>GSHMQQWVDCEFTGRDFRDEDLSRLHTERAMFSECDFSGVNLAESQHRGSAFRNCTFERTTLWHSTFAQCSMLGSVFVACRLRPLTLDDVDFTLAVLGGNDLRGLNLTGCRLRETSLVDTDLRKCVLRGADLSGARTTGARLDDADLRGATV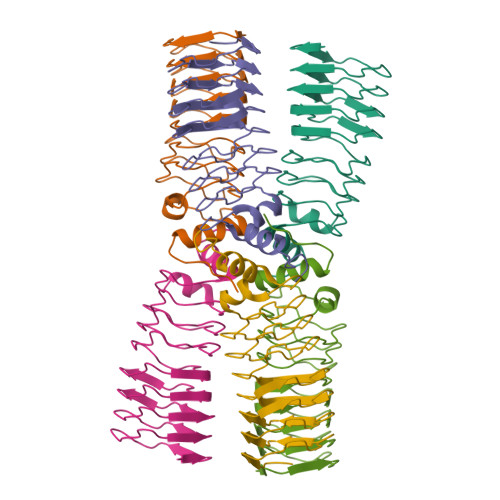DPVLWRTASLVGARVDVDQAVAFAAAHGLCLAGG[3x]> MEAGYAEIAAVQFNIAGDNDHKRQGVMEVTISNLFEGTLPAEGGIYDARMGTTDHHYKCITCSHQRKQCMGHPGILQMHAPVLQPLFIAEIRRWLRVICLNCGAPIVDLKRYEHLIRPKRLIEAASSQTEGKQCYVCKAVHPKIVKDSEDYFTFWADQQGKIDKLYPQIIREIFSRVTYDTVVKLGRSKNSHPEKLVLKAIQIPPISIRPGIRLGIGSGPQSFHDINNVIQYLVRKNLLIPKDLQIVRGQKIPLNIDRNLQTIQQLYYNFLLDSVSTTATQGGTGKRGIVMGARPAPSIMRRLPRKEGRIRKSLLGSQVWSISRSTICGNSDLHLDEVGYPISFARTLQVAETVQHYNINRLMPYFLNGKRQYPGCSRVYKQITQSVHDIEGLKQDFRLEVGDILYRDVVTGDVAFFNRQPSLERSSIGVHRIVVLENPKISTFQMNVSACAWYNADFDGDQMNLWVPWSVMSRVEAELLCSVRNWFISTKSSGPVNGQVQDSTVGSFLLTRTNTPMGKNVMNKLHAMGLFQTTQTDPPCFANYSPTDLLDGKSVVSMLLRQTPINYQRAPTWYSEVYAPYMHYNKQDISTQIRNGELIEGVLDKKAVGAGSSGGIYHLISRRYGPQQALKMIFATQQLALNYVRNAGFTVSTADMLLTPEAHQEVQEIINELLLESEEINNRLLHGDIMPPIGLTTHDFYEKLQLNALKFPDRILKPIMNSINPETNGLFQMVATGAKGSNPNMIHIMAGIGQIEINTQRIQPQFSFGRTLVYYPRFALEAQAYGFICNSYIAGLTSPEFIFGEMNGRFDLINKALSTSSTGYANRKAIFGLQSCIVDYYRRVSIDTRLVQQLYGEDGLDARQLETVRFETIMLSDQELEDKFKYTGIQSPLFEEEFSRLKKDRDKYRQIFLNVENFNFSQLLTDVRQVPVNVASIVKNILLSSTSGVLPFDEKSILQKYAMVKTFCKNLPYVFINNIQERLQTPIPVYLKRAASLMRMLIRIELATVKTLNITCEQMSAILDLIRLQYTQSLINYGEAVGILAAQSVSEPLTQYMLDSHHRSVAGGTNKSGIVRPQEIFSAKPVEAEQSSEMLLRLKNPEVETNKTYAQEIANSIELITFERLILQWHLLYETYSSTKKNVMYPDFASDVEWMTDFLENHPLLQPPEDIANWCIRLELNKTTMILKSISLESIINSLRAKHPNTYIMHSVENTASGIPIIIRIYLRESAFRRSTNTRMATDEKIAVNVVDKLLNSTIRGIPGIKNANVVKLMRHRVDAQGKLVRLDNIYAIKTNGTNIFGAMLDDNIDPYTIVSSSIGDTMELYGIEAARQKIISEIRTVMGDKGPNHRHLLMYADLMTRTGQVTSLEKAGLNAREPSNVLLRMALSSPVQVLTDAAVDSAVNPIYGIAAPTLMGSVPRIGTMYSDIIMDEKYITENYKSVDSLIDML;> MIDQKIFETTLNIDDPTNFCTNVEAHLLKELENIYVGKCFKNSFILNITGVIQRSPCFIMRTNNSGRGYMHVRFSAVVSYLNAFDLIAAVKIIKNDSNIILGESLLTEPVTIVIPSSESQNNVAEVGQIVPVQLANSSVYYIPGRQQASATGSIFIPKHTFSVYHVQEELTQEQALNLTKLVNIIEMLLESRSKKDFKQICFFEKLYYTYSISSDEILDLKIWKGPKGKEMSRLKPCNVLSFLYDALKNKNSSLGFWARPPNLLKSSPLAYQQDQNSFNATELPIICSAEVMFVTLLKEIINYLQFINDLCDTFNNEQLIKRHENIWMLIEQRKIGHDF;> MEEVITIAQIVHRGTDILSLNNEEIEALVDEIYSTLKGSNDIKNIRLIDFLFTLKDFVNHVRAEQSKLPDLSMPIEAYIRQLLVDPDVVPIVSEKKKELRVRPSTRKEIFLINGTHLAVPAEAPIEIYGLKLRLKTFSPQCFMRMAEIGSFSPETLGYVASGANLTNFIRVFMKCVDQETWKKNGEGVVVTTKENIIQFTHQYIELYKFLRSGGHSWLINRLAEEMVHRKLDREDQGSHISNIVETEEIEPEENIKRVIFFLKELSTMYSVSPVFTSGYMPLLYDLYRAGYLEVLWNPVEQKFLQHAEQREKEQMILQQVDMKLTEVITQARQ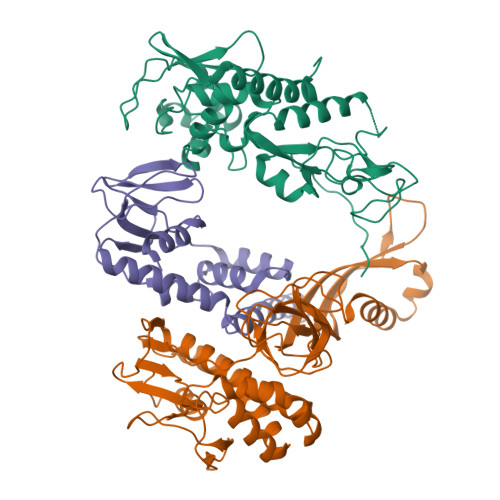YFKIMEEKIGRVQSDAIREILTMEGKVDDPNSILQEVIKACGKQEAELITTEYLNIKKQWELQEKNACAHLKLVKQLRSGLQYAELLKVLESIRVLYKEKNNTTNWNLCKACGFKLLCPHVDMLIQLQAAEASYDTMRTKLMKFSGINKEKENNQGLIYSYFCKICGEELAHFIQEDRTADVGIIGDLNSKLRVFIWQETMKACTFIHFGKLVDVKQFANIAVNVCLPLVYSIENIKKEEDYDPLTQLYAVIYIYAYILNLIYSSQKNKEFLTITIHGMKADSSLNAYVTFLLEKMMQQYSGIINQLSEITDQWIANNFREAFKKIIHQNGLQGLSVQDDTKVLLTEILLDPMYDYAATVARIDGSIPMHKPRTPKEAEYEFKTVIGRTPAELLSQKEFYDKIYTSKYRPDFTQLTRLNDIYFQEESLRVWWGGRDEEKTSTLIYLRAYELFLKYLQNAPNFNSELAEFKTYENAYGEQKALLAQQGFYNIFDPNTGRADQRTRLFEYKRLPISTLYDERGLPHKWTIYVYKAVDSSQKPAEIEVTRKDVIKKIDNHYALADLRCSVCHVLQHEVGQLNIKKVQTALKASLEFNTFYAFYESRCPKGGLHDFQDKKCVKCGLFTYIIYDHLSQPELVHDYYNNYKDQYDKEKMSIRSIQIKKDMTTPSTETQPKPPQEPWTFDYGKIIKTAKILDISPAVIEAIGAMEGRSYADIREGQGAPPPPTSMDDPRLMAVDSAVRIFLYNYNCLRHVSTFNKPPIHVERLVKHLSYEEKEDLEKVLPNVVNEYHTTFKHLRVTDPASALLYSIEFLCISFLTLYEIKEPSWVVNIVREFALTELNTIIQSEKLLSKPGAFNFMIFGEDFVCSGEDSSMDDISAYSSPGLFGEDIIDRLDDPFSIEDVDISLDVLDNLAPQ> KA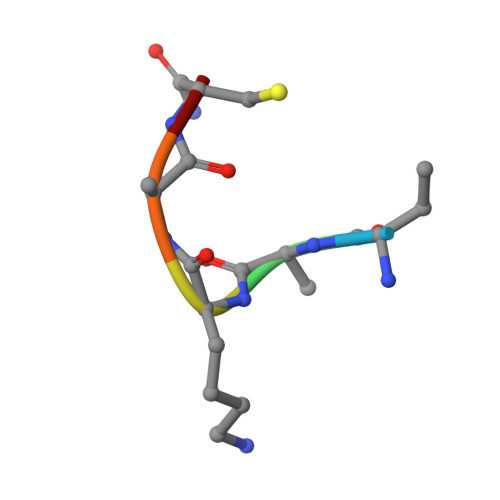KACX> MRGSHHHHHHGSNPYERGPDPTEDSIEAIRGPFSVATERVSSFASGFGGGTIYYPRETDEGTFGAVAVAPGFTASQGSMS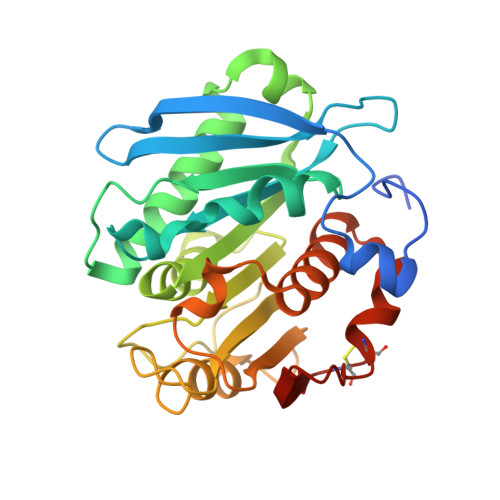WYGERVASQGFIVFTIDTNTRLDQPGQRGRQLLAALDYLVERSDRKVRERLDPNRLAVMGHSMGGGGSLEATVMRPSLKASIPLTPWNLDKTWGQVQVPTFIIGAELDTIAPVRTHAKPFYESLPSSLPKAYMELDGATHFAPNIPNTTIAKYVISWLKRFVDEDTRYSQFLCPNPTDRAIEEYRSTCPYKLN> FQSNAMKHCPITYEKISDQENYSQRGLHLLSPQLKNLSPL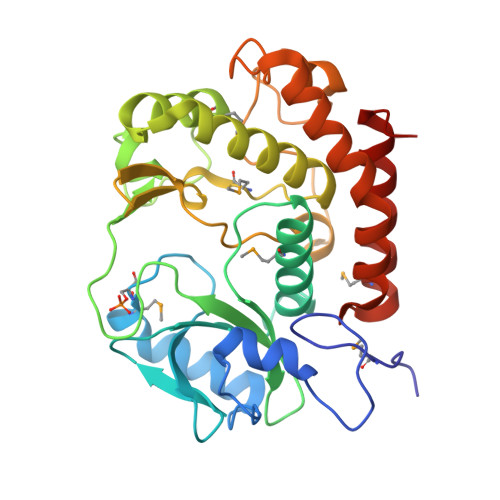DLSADEQRQEAIARVGKMSVQGVQKKLSAKLKIKEGCFEIVDQYGQYILKPQSDIYPELPENEAITMTLAKTIGLEVPVHGLVYSKDNSLTYFIKRFDRIGHNKKLALEDFAQLSGEDRHTKYKSSMEKVIAVIEQFCTFPKIEFVKLFKLTLFNFLVGNEDMHLKNFSLITKDRKISISPAYDLLNSTIAQKNTKEELALPLKGKKNNLTKSDFLKYFAIEKLGLNQNVIDGIVQEFHQVIPKWQELIGFSFLSQEMQEKYLELLEQRCKRLNFFD5-hydroxypyrazine-2,3-dicarboxylic acid | C6 H4 N2 O5 | 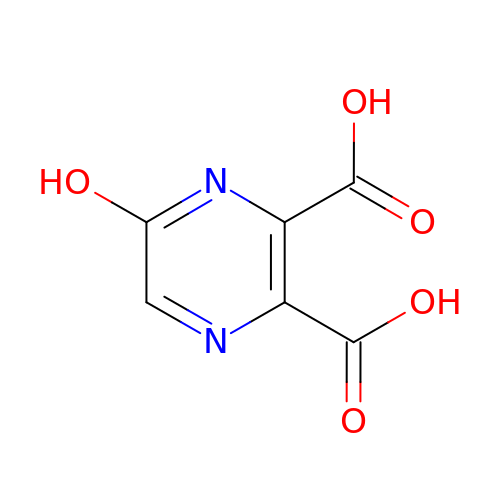IEFXAUUVZLXLNL-UHFFFAOYSA-N>MINEDFFIYEQLSHKKNLEQKGKNAFDEETEELVRQAKSGYHAFIEGINYDEVTKLDLNSSVAALEDYISIAKEIEKKHKMFNWRSDYAGSIIPEFLYRIVHVATVKAGLKPIFSTRNTIIEISGAAHREGLQIRRKNEDFALGFHEVDVKIASESHRVISLAVACEVKTNIDKNKLNGLDFSAERMKRTYPGSAYFLITETLDFSPDENHSSGLIDEIYVLRKQVRTKNRVQKAPLCPSVFAELLEDILEISYRASNVKGHVYDRLEGGKLIRV[2x];>[2x]MFNQFNPLVYTHGGKLERKSKKDKTASKVFEEFGVMEAYNCWKEASLCIQQRDKDSVLKLVAALNTYKDAVEPIFDS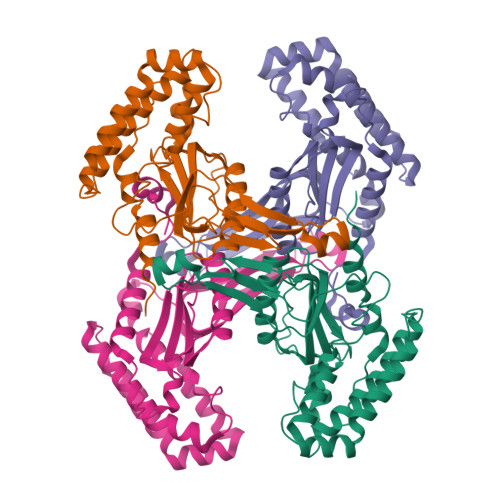RLNSAQEVLQPSILEEFFEYLFSRIDSIVGVNIPIRHPAKGYLSLSFNPHNIETLIQSPEYTVRAKDHDFIIGGSAKLTIQGHGGEGETTNIVVPAVAIECKRYLERNMLDECAGTAERLKRATPYCLYFVVAEYLKLDDGAPELTEIDEIYILRHQRNSERNKPGFKPNPIDGELIWDLYQEVMNHLGKIWWDPNSALQRGKVFNRP>MQSWYLLYCKRGQLQRAQEHLERQAVNCLAPMITLEKIVRGKRTA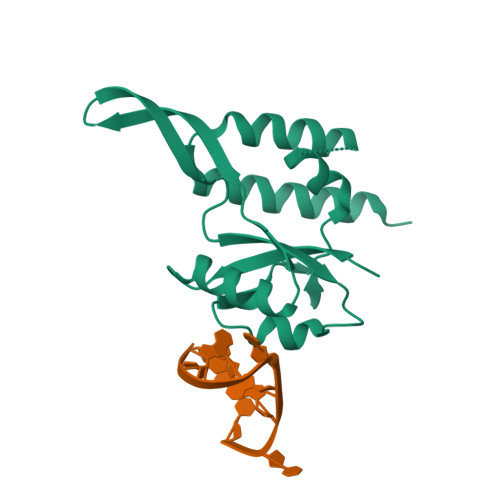VSEPLFPNYLFVEFDPEVIHTTTINATRGVSHFVRFGASPAIVPSAVIHQLSVYKPKDIVDPATPYPGDKVIITEGAFEGFQAIFTEPDGEARSMLLLNLINKEIKHSVKNTEFRKA[2x]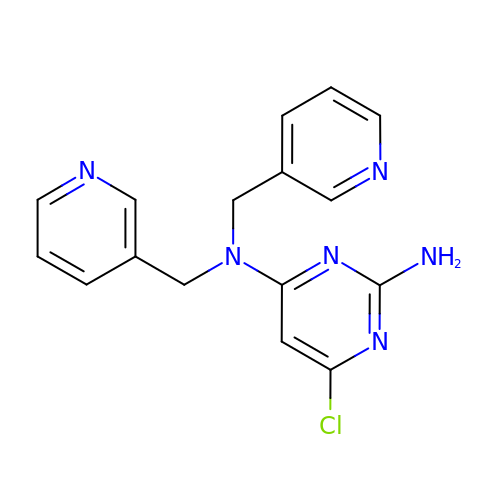6-chloro-N~4~,N~4~-bis[(pyridin-3-yl)methyl]pyrimidine-2,4-diamine | C16 H15 Cl N6 | JDMRUOFJLDXEIQ-UHFFFAOYSA-N>MGGSHHHHHHGMASMALKNKVQLITYPDSLGGNLKTLNDVLEKYFSDVFGGVHILPPFPSSGDRGFAPITYSEIEPKFGTWYDIKKMAENFDILLDLMVNHVSRRSIYFQDFLKKGRKSEYADMFITLDKLWKDGKPVKGDIEKMFLRRTLPYSTFKIEETGEEEKVWTTFGKTDPSEQIDLDVNSHLVREFLLEVFKTFSNFGVKIVRLDAVGYVIKKIGTSCFFVEPEIYEFLDWAKGQAASYGIELLLEVHSQFEVQYKLAERGFLIYDFILPFTVLYTLINKSNEMLYHYLKNRPINQFTMLDCHDGIPVKPD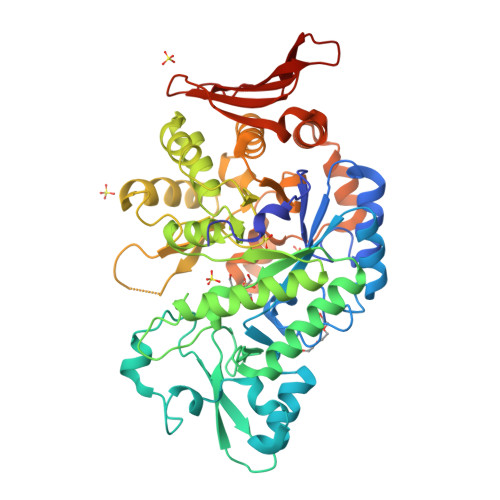LDGLIDTKKAKEVVDICVQRGANLSLIYGDKYKSEDGFDVHQINCTYYSALNCDDDAYLAARAIQFFTPGIPQVYYVGLLAGVNDFEAVKKTKEGREINRHNYGLKEIEESVQKNVVQRLLKLIRFRNEYEAFNGEFFIEDCRKDEIRLTWKKDDKRCSLFIDLKTYKTTIDYINENGEEVKYLV[2x]> SNAEVSVGKATDIYAVNGTEILLPCTFSSAFGFEDLHFRWTYNSSDAFKILTEGTVKNEKSDPKVTLKDDDRITLVGSTKEKMNNISIVLRDLEFSDTGKYTCHVKNP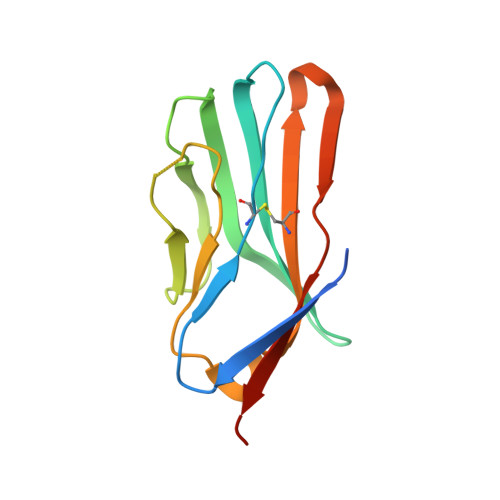KENNLQHHATIFLQVVDRLEE> MAHHHHHHGVRHVALSVDASEWRQPVFKQKVLAILRRLHVPRWSSPLLTPTNIHLQKVSGALTNAVFFVSFNPAPNPTSPSESPLLTPTIPPSDPSHPPPLTPEQYPHTLLFRVYGPSSDALISRSEELRILHVLSTQYGIGPRVFGTFTNGRVEEFFPSRALTAQELRDPIISRGIARRMRELHSVDLRRLGYEQGRATEPALWICLKEWSEAAEDVISSLTALGGTLEAWVERFSLHRIREEVTIYRNFVESQSGKGNGVVFAHNDTQYGNLLRLDVELPPNTPEHCRYIVIDFEYASPNPRGYDIANHFHEWRANYHHPTHSHSLIPHFPYPTPIQREDFYRSYLSVEVDGRNGEEVVGKRKDVPADKVAALEHEVRIWSPGCSINWALWGLVQAEEQVC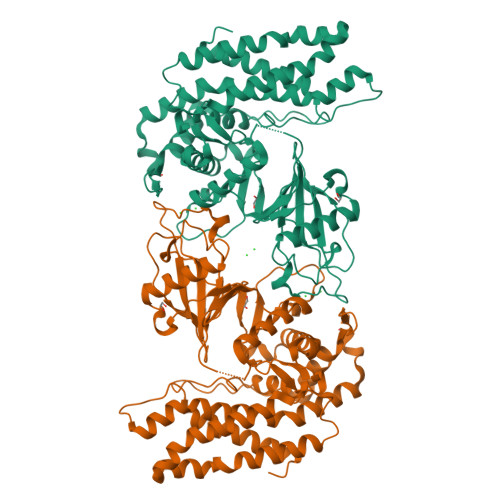ALATKKEGYVPEFDYLSYAAERLEMFRDEAKKLGVPL> THRLITLADHICQIITQD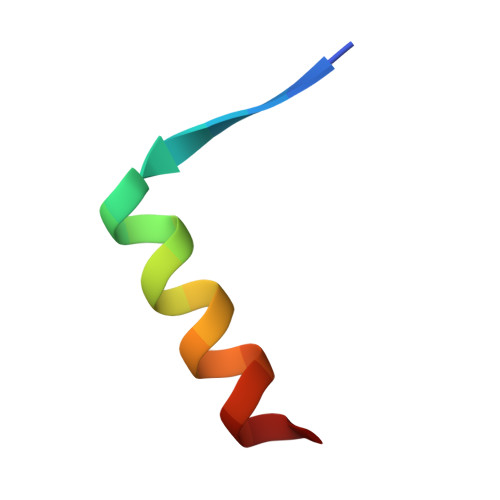FAR>VEFDRADILYNIRQTSRPDVIPTQRDRPVAVSVSLKFINILEVNEITNEVDVVFWQQTTWSDRTLAWNSSHSPDQVSVPISSLWVPDLAAYNAISKPEVLTPQLARVVSDGEVLYMPSIRQRFSCDVSGVDTESGATCRIKIGSWTHHSREISVDPTTENSDDSEYFSQYSRFEILDVTQKKNSVTYSCCP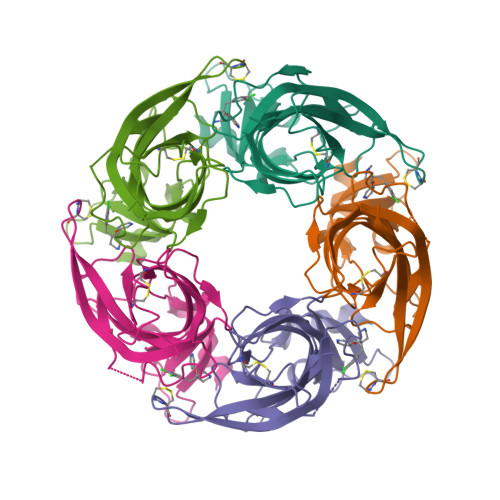EAYEDVEVSLNFRKKGRSEIL[5x]>[2x]MSIKIRDFGLGSDLISLTNKAGVTISFTNLGARIVDWQKDGKHLILGFDSAKEYLEKDAYPGATVGPTAGRIKDGLVKISGKDYILNQNEGPQTLHGGEESIHTKLWTYEVTDLGAEVQVKFSLVSNDGTNGYPGKIEMSVTHSFDDDNKWKIHYEAISDKDTVFNPTGNVYFNLNGDASE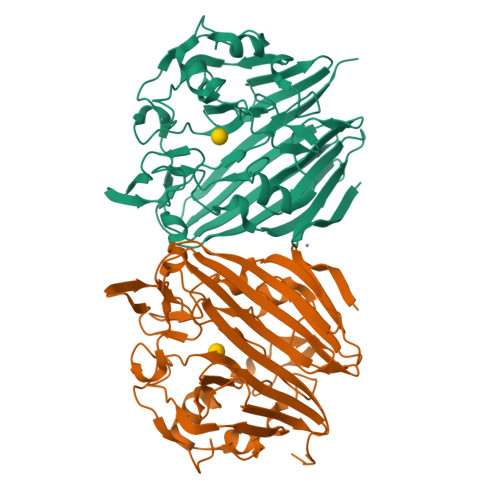SVENHGLRLAASRFVPLKDQTEIVRGDIVDIKNTDLDFRQEKQLSNAFNSNMEQVQLVKGIDHPFLLDQLGLDKEQARLTLDDTSISVFTDQPSIVIFTANFGDLGTLYHEKKQVHHGGITFECQVSPGSEQIPELGDISLKAGEKYQATTIYSLHTKLEHHHHHH> TFAYKIDGNEVIFTLWAPYQKSVKLKVLEKGLYEMERDEKGYFTITLNNVKVRDRYKYVLDDASEIPDPASRYQPEGVHGPSQIIQESKEFNNETFLKKEDLIIYEIHVGTFTPEGTFEGVIRKLDYLKDLGITAIEIMPIAQFPGKRDWGYDGVYLYAVQNSYGGPEGFRKLVDEAHKKGLGVILDVVYNHVGPEGNYMVKLGPYFSQKYKTPWGLTFNFDDAESDEVRKFILENVEYWIKEYNVDGFRLDAVHAIIDTSPKHILEEIADVVHKYNRIVIAESDLNDPRVVNPKEKCGYNIDAQWVDDFHHSIHAYLTGERQGYYTDFGNLDDIVKSYKDVFVYDGKYSNFRRKTHGEPVGELDGCNFVVYIQNHDQVGNRGKGERIIKLVDRES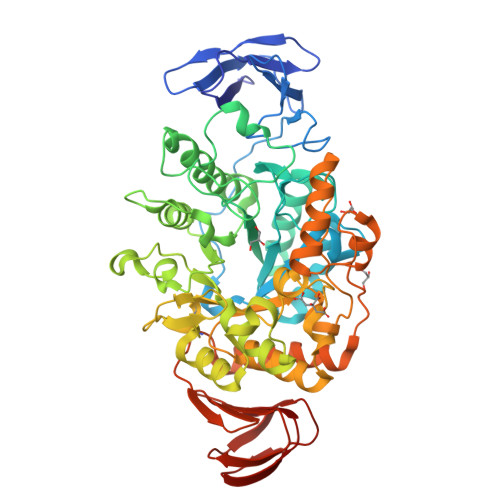YKIAAALYLLSPYIPMIFMGEEYGEENPFYFFSDFSDSKLIQGVREGRKKENGQDTDPQDESTFNASKLSWKIDEEIFSFYKILIKMRKELSIACDRRVNVVNGENWLIIKGREYFSLYVFSKSSIEVKYSGTLLLSSNNSFPQHIEEGKYEFDKGFALYKL>XGEIAQTIKEIAKTIKEIAYTI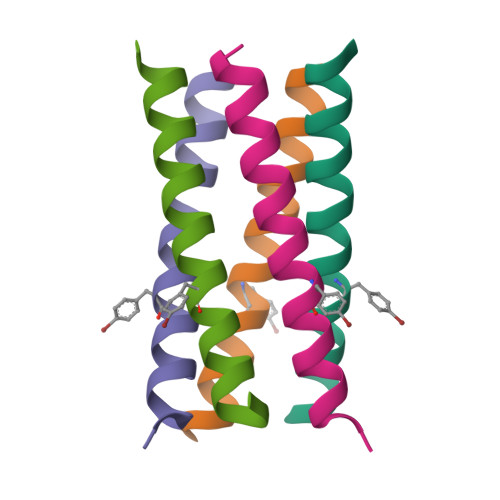KEIAQTIKGX[10x]>[2x]MGSSHHHHHHSSGENLYFQGHMESALAVPRLPPHDPGTPVLSVVDMHTGGEPLRIVLAGCPEVSGPTLLAKRRYMRQHLDHVRRRLMFEPRGHRDMYGAVLVPSELPDAHLGVLFLHNEGYSSMCGHAVLALGRFALDFGLVPAPPAGTREARVNIHCPCGLVTAFVACEDGRSHGPVRFHSVPAFVLATDLMVDVPGHGKVMVDIAYGGAFYAFVTAEKLGLDICSAKTRDLVDAASAVTEAVKAQFKINHPDSEDLAFLYGTILTDGKDAYTKEPTTNICVFADEQVDRSPTGSGVTARIALQYHKGLLELNQMRAFKSSATGSVFTGKAVREAKCGDFKAVIVEVSGQAHYTGTASFIIEDDDPLRDGFLLK

hL3HYPDH was first discovered by Visser and colleagues who identified, through sequence alignments between orthologs of the proline racemases family, the human protein C14orf149 (named after its gene locus and later named hL3HYPDH) which lacked racemase activity but exhibited instead proline dehydratase activity, converting trans-3-hydroxy-l-proline (T3LHyp) into Δ1-pyrroline-2-carboxylate (Pyr2C). hL3HYPDH is involved in the metabolism of hydroxyproline (Hyp), a non-standard amino acid present in the cell wall components of plants and in mammalian collagen and deriving from the post-translational modification of proteins by prolyl hydroxylase enzymes. While T4LHyp is metabolised following distinct degradative pathways in mammals and bacteria, the T3LHyp metabolic pathway is conserved in bacteria, plants and mammals, and involves a T3LHyp dehydratase (EC 4.2.1.77) which removes the hydroxyl group of T3LHyp without the intervention of a cofactor, leading to the formation of Δ2-pyrroline-2-carboxylate. Besides its role in the dietary hydroxyproline metabolism, hL3HYPDH has been also identified among the interferon-stimulated genes (ISGs) triggered by virus infection and showing antiviral activities.

Crystal screening and optimization of recombinant hL3HYPDH in absence and in presence of the substrate or the transition-state analogue pyrrole-2-carboxylic acid (PYC) produced crystals that best diffracted at 3.0 Å. The final hL3HYPDH model was reliably built between amino acids 10–354 (for chain A) and 4–354 (for chain B) except for residues 150–152 and 227–239 of both chains due to the missing or poor-quality electron density. Although hL3HYPDH crystallized in presence of the substrate T3LHyp or the transition state analogue PYC, examination of the catalytic centres of the two monomers did not reveal electron density attributable to these molecules. Unlike the structures of tlT3LHypD and of tcProR that both showed a closed conformation for the ligand-complexed monomer and an open conformation of the ligand-free monomer, both hL3HYPDH monomers exhibited an open conformation, consistent with the absence of ligands in both catalytic sites. However, structural alignment between the predicted and experimental hL3HYPDH models revealed a significant difference in the conformation of the mobile domains, being the experimental and the predicted structure in the open and closed conformation, respectively. Moreover, a hydrogen bond between Asp98 and Gln267 (3.4 Å) further stabilizes the open conformation; however, this interaction is lost in the closed state, as observed in the predicted structure, where Tyr76 and Tyr241 engage in an H-bond (3.2 Å). In hL3HYPDH, residues Met103 and Ser275 play a stabilizing role of the open conformation through hydrogen bonding of the hydroxy group of Ser275 and the sulphur of Met103 (3.0 Å), locking Met103 in an extended conformation and protruding it toward the free substrate-binding site.>[2x]DVSGTVCLSALPPEATDTLNLIAS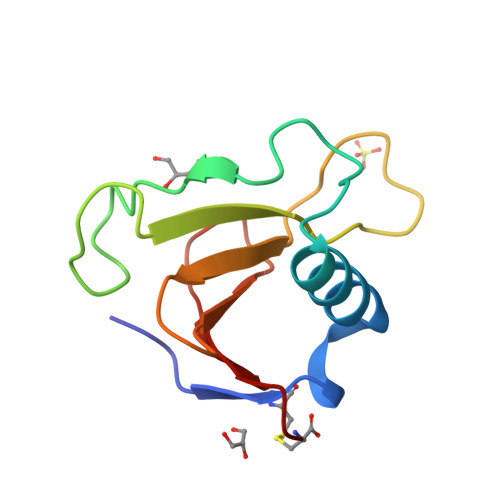DGPFPYSQDGVVFQNRESVLPTQSYGYYHEYTVITPGARTRGTRRIITGEATQEDYYTGDHYATFSLIDQTC> MSPILGYWKIKGLVQPTRLLLEYLEEKYEEHLYERDEGDKWRNKKFELGLEFPNLPYYIDGDVKLTQSMAIIRYIADKHNMLGGCPKERAEISMLEGAVLDIRYGVSRIAYSKDFETLKV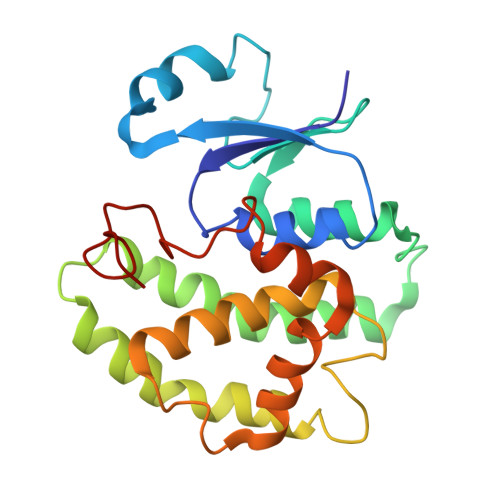DFLSKLPEMLKMFEDRLCHKTYLNGDHVTHPDFMLYDALDVVLYMDPMCLDAFPKLVCFKKRIEAIPQIDKYLKSSKYIAWPLQGWQATFGGGDHPPK> SNAETIEIIKDLFEHLCGVRVHRTYEDDTGLWFDTSQGSKNGIMDYKLGFV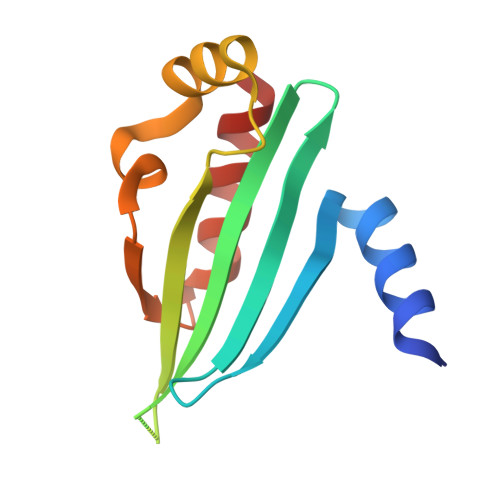KSQAENTTEVDTEVIYVPLLKQRTAEELQELQKKLPDYLFETLSFPLRSLNQFYIKMSKSLNKKV> K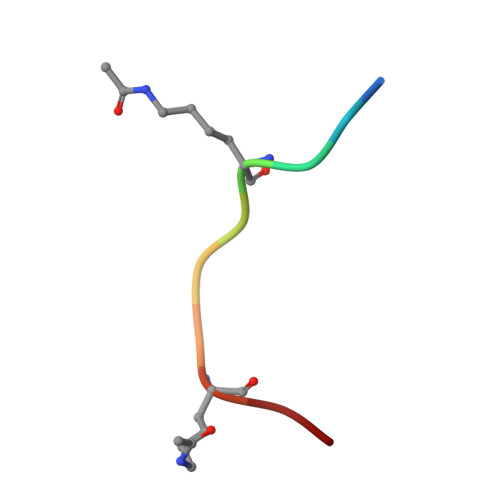GGKGLGKGG Mal, which is also identified as the TIR domain-containing adaptor protein (TIRAP), is essential for the TLR4 and TLR2 signaling pathways. Mal acts as a bridge adaptor to recruit the MyD88 molecule to the activated TLR4 dimer on the plasma membrane. The C-terminus (residues 80–221) of Mal, referred to as Mal-TIR, is the TIR domain and is required for interactions with TLR4, TLR2 and MyD88. The overall structure of Mal-TIR consists of a central five-stranded parallel sheet (βA-βE) surrounded by four helices (αA, αC-αE) on both sides.

Among these, D96N, E132K, R143Q and E190D have been reported to cause a loss of function in Mal. The D96N mutation has also been shown to impair recruitment of MyD88 to the plasma membrane and to influence the post-translational modification of Mal. To further understand the molecular mechanism underlying these associations in the Mal-TIR mutants D96N and S180L, we determined the crystal structures of these mutants. These structures showed that neither mutation interferes with the overall structure of the TIR domain. We also found that the surface electronic potential map and hydrophobicity of the Mal-TIR D96N mutant does not obviously differ from that of the wild-type protein. Our observations are inconsistent with the recent conclusion based on an in silico model that the D96N mutant fails to associate directly with MyD88 because this mutation affects the distribution of negative charge on the MyD88 binding site of Mal. Our direct binding assay also showed that Mal-TIR D96A retains the same binding affinity to MyD88-TIR and TLR4-TIR as that observed in wild type, and the D96N mutant is capable of binding with MyD88-TIR. Additionally, the D96E mutant, which retains the negative charge at that position, results in the complete loss of NF-κB activation. Thus, we conclude that the loss of function in Mal D96N is not caused by interference with the interaction between Mal and MyD88 but instead by another mechanism, such as altered post-translational modification of Mal. We also showed that D96N and L165A can bind normally to MyD88-TIR.

> GPGSSRWSKDYDVCVCHSEENLVAAQDLVSYLEGSTASLRCFLQLRDATPGGAIVSELCQALSSSHCRVLLITPGFLQDPWCKYQMLQALTEAPGAEGCTIPLLSGLSRAAYPPELRFMYYVDGRGPDGGFRQVKEAVMRYLQTLS>[2x]MGSSHHHHHHSAG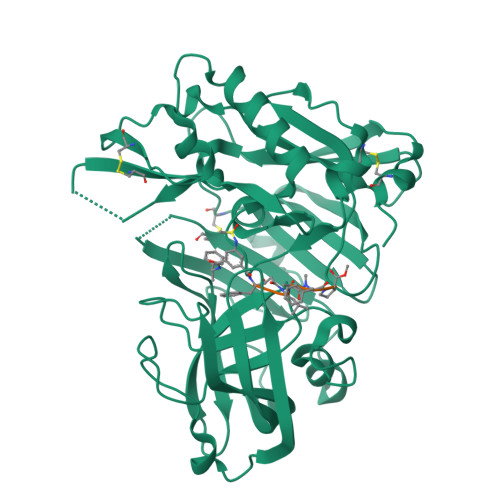ENLYFQGTLPRETDEEPEEPGRRGSFVEMVDNLRGKSGQGYYVEMTVGSPPQTLNILVDTGSSNFAVGAAPHPFLHRYYQRQLSSTYRDLRKGVYVPYTQGAWAGELGTDLVSIPHGPNVTVRANIAAITESDKFFINGSNWEGILGLAYAEIARPDDSLEPFFDSLVKQTHVPNLFSLQLCGAGFPLNQSEVLASVGGSMIIGGIDHSLYTGSLWYTPIRREWYYEVIIVRVEINGQDLKMDCKEYNYDKSIVDSGTTNLRLPKKVFEAAVKSIKAASSTEKFPDGFWLGEQLVCWQAGTTPWNIFPVISLYLMGEVTNQSFRITILPQQYLRPVEDVATSQDDCYKFAISQSSTGTVMGAVIMEGFYVVFDRARKRIGFAVSACHVHDEFRTAAVEGPFVTLDMEDCGYNIPQTDEST> MSAQVMLEDMARKYAILAVKADKEGKVEDAITYYKKAIEVLSQIIVLYPESVARTA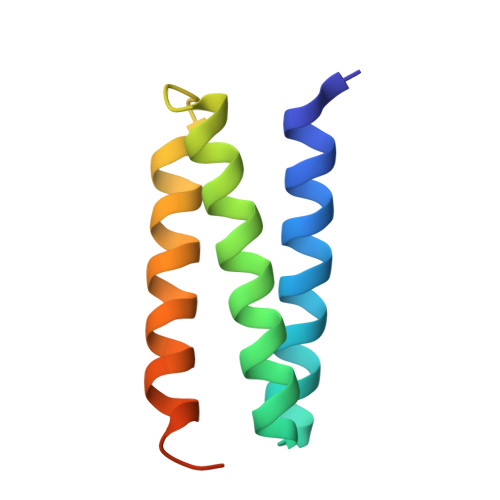YEQMINEYKKRISYLEKVLPASSDGSG>[4x]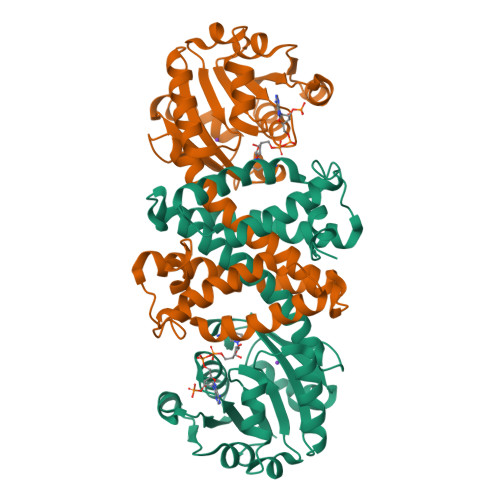MKPSISVLGTGRMGSALARALLQAGYRTVVWNRTSEKAEPLAALGATVAPTVRQAIDASGIVIVNVSDYAATSTLLRASDVTPGLRGKLIVELTSGTPEGARETSQWTAAHGARYLDGAILATPDFIGTDAGTILLSGALEPFAANEDVFRALGGNVQHIGTEPGLANALDSAVLALMWGALFGGLHAIAVCRAEEIDLGELGRQWAATAPVVEGLVADLIKRTSAGRFVSDAETLSSISPHYGAFQHLKELMEARRIDRTVVDGYDAIFRRAIASGHLHDDFAALSQFMGKAEQP>[12x]MKTPTIPTLLGPDGMTSLREYAGYHGGGSGFGGQLRSWNPPSESVDAALLPNFTRGNARADDLVRNNGYAANAIQLHQDHIVGSFFRLSHRPSWRYLGIG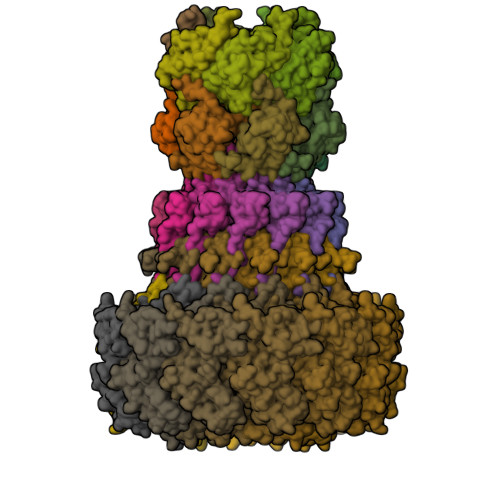EEEARAFSREVEAAWKEFAEDDCCCIDVERKRTFTMMIREGVAMHAFNGELFVQATWDTSSSRLFRTQFRMVSPKRISNPNNTGDSRNCRAGVQINDSGAALGYYVSEDGYPGWMPQKWTWIPRELPGGRASFIHVFEPVEDGQTRGANVFYSVMEQMKMLDTLQNTQLQSAIVKAMYAATIESELDTQSAMDFILGANSQEQRERLTGWIGEIAAYYAAAPVRLGGAKVPHLMPGDSLNLQTAQDTDNGYSVFEQSLLRYIAAGLGVSYEQLSRNYAQMSYSTARASANESWAYFMGRRKFVASRQASQMFLCWLEEAIVRRVVTLPSKARFSFQEARSAWGNCDWIGSGRMAIDGLKEVQEAVMLIEAGLSTYEKECAKRGDDYQEIFAQQVRETMERRAAGLKPPAWAAAAFESGLRQSTEEEKSDSRAA;>[6x]MKHTELRAAVLDALEKHDTGATFFDGRPAVFDEADFPAVAVYLTGAEYTGEELDSDTWQAELHIEVFLPAQVPDSELDAWMESRIYPVMSDIPALSDLITSMVASGYDYRRDDDAGLWSSADLTYVITYEM;>[12x]MTRQEELAAARAALHDLMTGKRVATVQKDGRRVEFTATSVSDLKKYIAELEVQTGMTQRRRGPAGFYV;>[6x]MADFDNLFDAAIARADETIRGYMGTSATITSGEQSGAVIRGVFDDPENISYAGQGVRVEGSSPSLFVRTDEVRQLRRGDTLTIGEENFWVDRVSPDDGGSCHLWLGRGVPPAVNRRR Siah1 (seven-in-absentia homologue 1) is an E3 ligase belonging to the RING (really interesting new gene) domain family. It acts as a scaffolding protein and interacts with a variety of different substrates for ubiquitination and subsequent degradation. Siah1 functions in Ras, DNA-damage and hypoxia signalling pathways, and is implicated in various cancers. The SBD forms a dimerization interface with its counterpart from the partner subunit to create a Z-shaped structure.

Two isomorphous crystal structures of Siah1 were determined at 1.95 and 1.58 Å resolution. There are two molecules per asymmetric unit, labelled chains A and B, and they form a dimer consistent both with the observation that a single species of approximate mass 39 kDa was noted during size-exclusion chromatography purification and with published structures of Siah1. The electron-density map was very well defined in the 1.58 Å resolution structure, apart from one loop region (Tyr199–Gly201 in chain A and Lys198–Tyr199 in chain B), and these residues were excluded from the model. A Ramachandran plot shows that 97.4% of the residues in the high-resolution structure are located in the most favoured region, with no outliers. The degree of NCS is more highly conserved in the high-resolution structure, in which the superposition of chain A on chain B (171 Cα positions) results in an r.m.s.d. of 1.36 Å. Superposition of the two new structures on each other gives r.m.s.d. values of 0.80 and 4.89 Å for chains A (175 Cα atoms) and B (164 Cα atoms), respectively. The high value again occurs owing to a difference in the position of the N-terminal zinc-finger subdomain in the two structures. The result is that the Zn2+ ions are displaced by about 14.5 Å when the structures are superposed. The overall molecular packing in each lattice remains well conserved and it is simply that there is space that allows the N-­terminal zinc finger of the B chain to adopt a position where it can either interact with a molecule at 1 − x + ½, y + ½, −z + ½ as in the highest resolution structure or interact with a molecule at 1 − x, 1 − y, z as in the case of the lower resolution structure. The notable conformational flexibility of the N-terminal zinc-finger subdomain may contribute to its role in the biological function by adapting its position to assist in interactions with distinct substrate proteins.

>GHMANSVLFPCKYASSGCEITLPHTEKADHEELCEFRPYSCPCPGASCKWQGSLDAVMPHLMHQHKSITTLQGEDIVFLATDINLPGAVDWVMMQSCFGFHFMLVLEKQEKYDGHQQFFAIVQLIGTRKQAENFAYRLELNGHRRRLTWEATPRSIHEGIATAIMNSDCLVFDTSIAQLFAENGNLGINVTISMC[2x]>[2x]SIQKIWAREILDSRGNPTVEVDLYTAKGLFRAAVPSGAST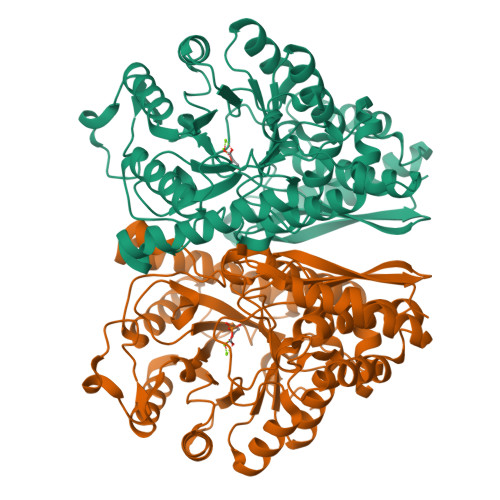GIYEALELRDGDKQRYLGKGVLKAVDHINSTIAPALISSGLSVVEQEKLDNLMLELDGTENKSKFGANAILGVSLAVCKAGAAERELPLYRHIAQLAGNSDLILPVPAFNVINGGSHAGNKLAMQEFMILPVGAESFRDAMRLGAEVYHTLKGVIKDKYGKDATNVGDEGGFAPNILENSEALELVKEAIDKAGYTEKIVIGMDVAASEFYRDGKYDLDFKSPTDPSRYITGDQLGALYQDFVRDYPVVSIEDPFDQDDWAAWSKFTANVGIQIVGDDLTVTNPKRIERAVEEKACNCLLLKVNQIGSVTEAIQACKLAQENGWGVMVSHRSGETEDTFIADLVVGLCTGQIKTGAPCRSERLAKYNQLMRIEEELGDEARFAGHNFRNPSVLHHHHHH> RCELKLIASP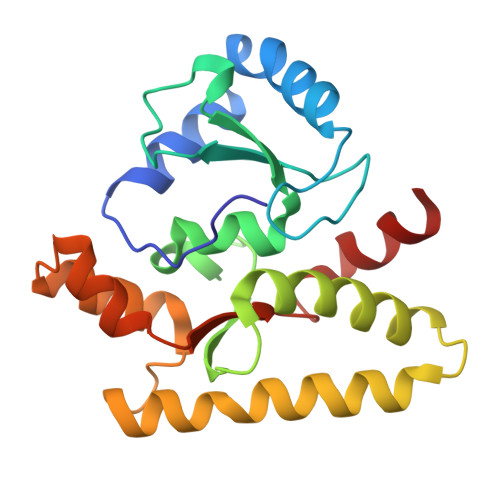GSWRLYSARKIDARFKSYEQKIFQRDRYTCQFCGFQAALYQDIVNLDGDYTNNRLSNLVTACCFCAQCFFVESVGVGGYGGGTLIYLPELTQAELNSLCHVLFCAITNDTGYKSSAQNIYRSFKFRSQIVEEKFGEGTSDPAIFGQLMIDSGVNSEEIREKLFKNIRLLPSRAKFRKQIEKWAAA>DYKDDDDKLHSQANLMRLKSDLFNRSPMYPGPTKDDPLTVTLGFTLQDIVKADSSTNEVDLVYWEQQRWKLNSLMWDPNEYGNITDFRTSAADIWTPDITAYSSTRPVQVLSPQIAVVTHDGSVMFIPAQRLSFMCDPTGVDSEEGATCAVKFGSWVYSGFEIDLKTDTDQVDLSSYYASSKYEILSATQTRQVQHYSCCPEPYIDVNLVVKFRERRAGN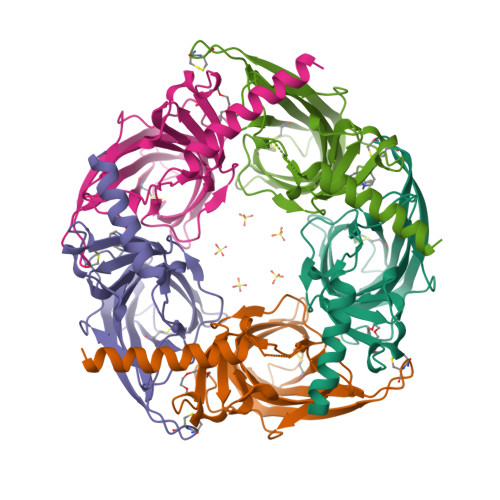GFFRNLFDSR[10x]> MAISLATKAATDALKVNRAPVGVEPQEVHKWLQSFNWDFKENRTKYPTKYHMANETKEQFKVIAKEYARMEAAKDERQFGTLLDGLTRLGAGNKVHPRWGETMKVISNFLEVGEYNAIAASAMLWDSATAAEQKNGYLAQVLDEIRHTHQCAFINHYYSKHYHDPAGHNDARRTRAIGPLWKGMKRVFADGFISGDAVECSVNLQLVGEACFTNPLIVAVTEWASANGDEITPTVFLSVETDELRHMANGYQTVVSIANDPASAKFLNTDLNNAFWTQQKYFTPVLGYLFEYGSKFKVEPWVKTWNRWVYEDWGGIWIGRLGKYGVESPASLRDAKRDAYWAHHDLALAAYAMWPLGFARLALPDEEDQAWFEANYPGWADHYGKIFNEWKKLGYEDPKSGFIPYQWLLANGHDVYIDRVSQVPFIPSLAKGTGSLRV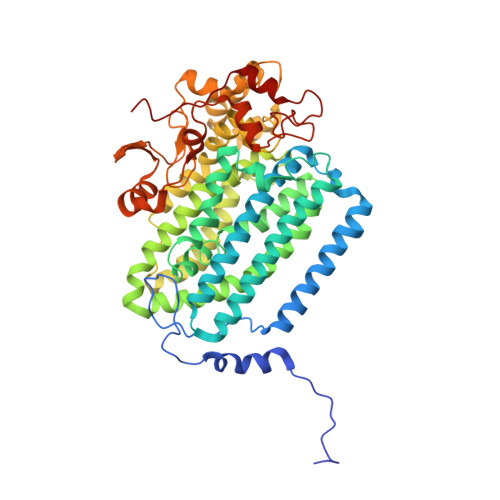HEFNGKKHSLTDDWGERQWLIEPERYECHNVFEQYEGRELSEVIAEGHGVRSDGKTLIAQPHTRGDNLWTLEDIKRAGCVFPDPLAKF>TTVYYDQDVKTDALQGKKIAVVGYGSQGHAHAQNLKDNGYDVVIGIRPGRSFDKAKEDGFDVFPVAEAVKQADVIMVLLPDEIQGDVYKNEIEPNLEKHNALAFAHGFNIHFGVIQPPADVDVFLVAPKGPGHLVRRTFVEG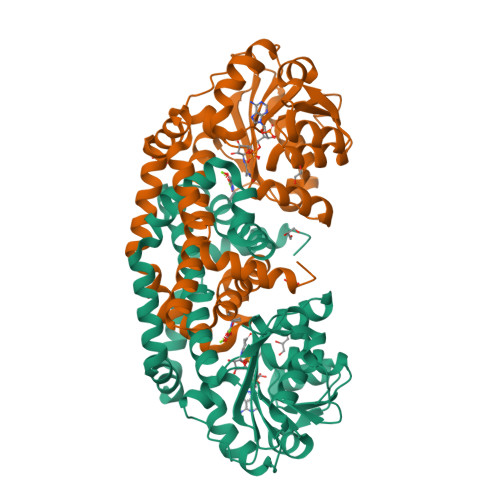SAVPSLFGIQQDASGQARNIALSYAKGIGATRAGVIETTFKEETETDLFGEQAVLCGGVSKLIQSGFETLVEAGYQPELAYFEVLHEMKLIVDLMYEGGMENVRYSISNTAEFGDYVSGPRVITPDVKENMKAVLTDIQNGNFSNRFIEDNKNGFKEFYKLREEQHGHQIEKVGRELREMMPFIKSKSIEKHHHHHH[2x]>[2x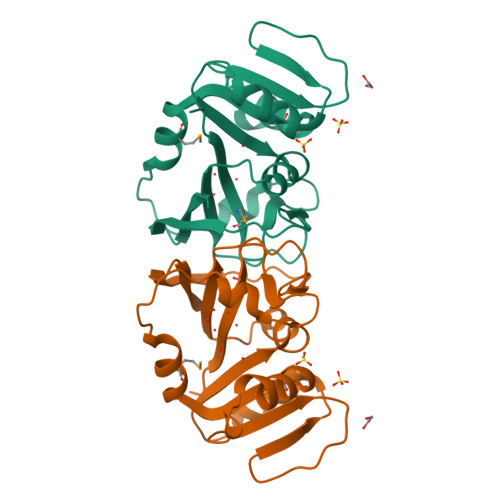]GMARKVILFIAMSIDNYIADDQGAVDWLEKNVHGTESDDSYEKMYSKIDTVIMGRTTYEQVTQKLSPEKYVYADRQTYIVTSHLGEDTDKIKYWKQSPVELVKRIQKEKGKDVWIVGGAKIIDPLVQANLIDTYILTTVPIFLGSGIRLFDRLEEQVPVRLIDVYQKNELVYSIYQRG> MGKAEAINEIQKAVASNKVIVYSKTYCPY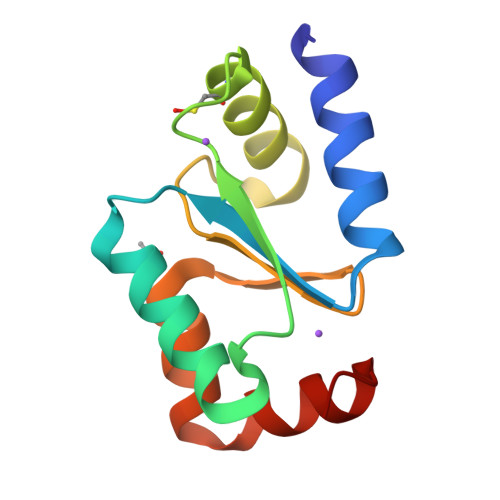CVKAKNALNQFIAGKYTVVELENRADCDAMQDALLDITGGRSVPRVFINGKFLGGGDDTAAAASNGTLEKLLQEAGAL>[2x]MGSSHHHHHHSSGRENLYFQGHMRTVSHPTPLRRAPVQRRSAERLTRILDACADLLDEVGYDALSTRAVALRADVPIGSVYRFFGNKRQMADALAQRNLERYAERVTERLTEAGDGGWRGAL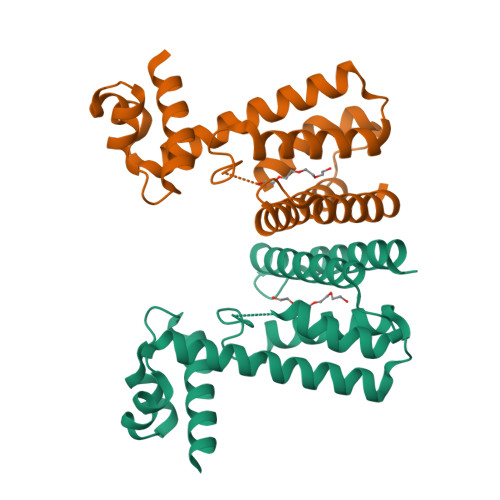DTVLDEYLAMKRTAPGFSLIDFGNQIPVGDRHAVPNHRVAERLTELLSGYLGRRPDDDLRRVFLVAVETADTLVQLAFRVAPDGDEKIIEEARELLRAYLGRVLDGS> MQVKPCTPEFYQTHFQLAYRLQSRPRGLALVLSNVHFTGEKELEFRSGGDVDHSTLVTLFKLLGYDVHVLCDQTAQEMQEKLQNFAQLPA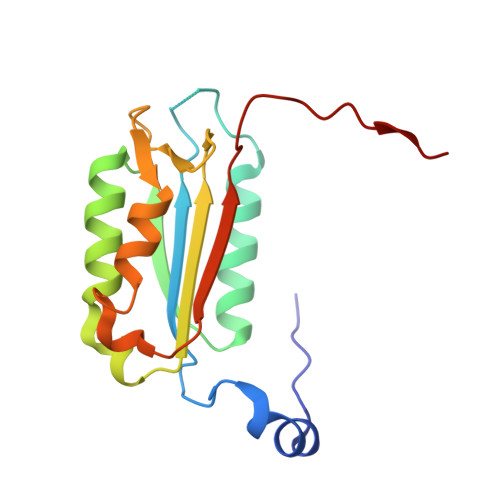HRVTDSCIVALLSHGVEGAIYGVDGKLLQLQEVFQLFDNANCPSLQNKPKMFFIQACRGDETDRGVDQQD> MASVIEQCQVVPSPGSATELTLPLTYFDHVWLAFHRMRRILFYKLPISRPDFVQTIIPTLKDSLSLTLKYYLPLAGNVACPQDWSGYPELRYVTGNSVSVIFSESDMDFNYLIGYHPRNTKDFYHFVPQLAEPKDAPGVQLAPVLAIQVTLFPNHGISIGFTNHHVAGDGATIVKFVRAWALLNKFGGDEQFLANEFIPFYDRSVIKDPNGVGMSIWNEMKKYKHMMKMSDVVTPPDKVRGTFIITRHDIGKLKNLVLTRRPKLTHVTSFTVTCAYVWTCIIKSEAATGEEIDENGMEFFGCAADCRAQFNPPLPPSYFGNALVGYVARTRQVDLAGKEGFTIAVELIGEAIRKRMKDEEWILSGSWFKEYDKVDAKRSLSVAGSPKLDLYA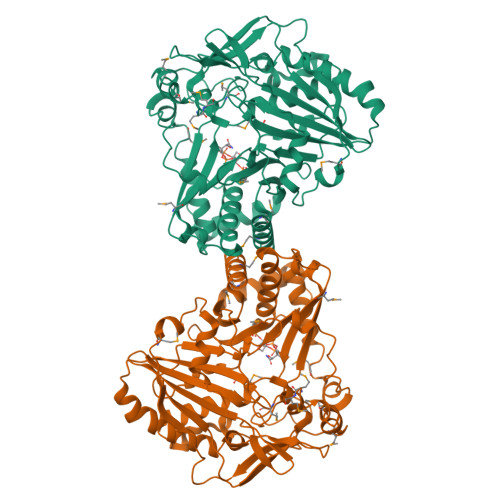ADFGWGRPEKLEFVSIDNDDGISMSLSKSKDSDGDLEIGLSLSKTRMNAFAAMFTHGISFL>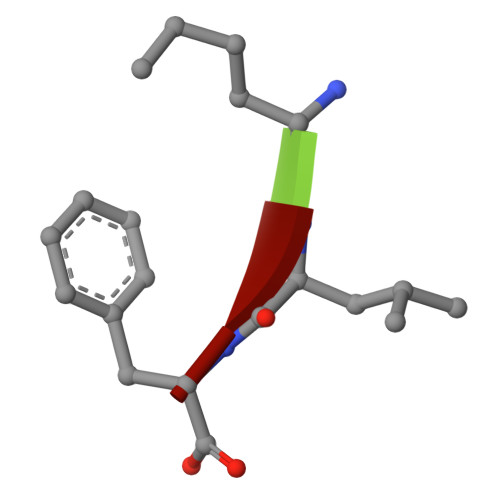 LLF>MSPPVYSDISRNINDLLNKDFYHATPAAFDVQTTTANGIKFSLKAKQPVKDGPLSTNVEAKLNDKQTGLGLTQGWSNTNNLQTKLEFANLTPGLKNELITSLTPGVAKSAVLNT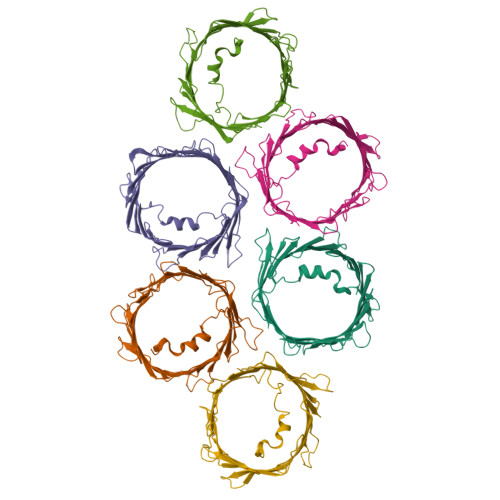TFTQPFFTARGAFDLCLKSPTFVGDLTMAHEGIVGGAEFGYDISAGSISRYAMALSYFAKDYSLGATLNNEQITTVDFFQNVNAFLQVGAKATMNCKLPNSNVNIEFATRYLPDASSQVKAKVSDSGIVTLAYKQLLRPGVTLGVGSSFDALKLSEPVHKLGWSLSFDA[6x]>[4x]GLSSSPSEILQELGKGSTHPQPGVSPPAAPAAPGPKDGPGETDAFGNSEGKELVASGENKIKQGLLPSLEDLLFYTIAEGQEKIPVHKFITALKSTGLRTSDPRLKECMDMLRLTLQTTSDGVMLDKDLFKKCVQSNIVLLTQAFRRKFVIPDFMSFTSHIDELYESAKKQSGGK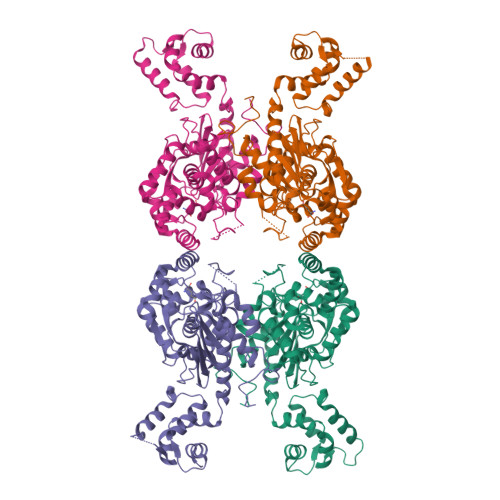VADYIPQLAKFSPDLWGVSVCTVDGQRHSTGDTKVPFCLQSCVKPLKYAIAVNDLGTEYVHRYVGKEPSGLRFNKLFLNEDDKPHNPMVNAGAIVVTSLIKQGVNNAEKFDYVMQFLNKMAGNEYVGFSNATFQSERESGDRNFAIGYYLKEKKCFPEGTDMVGILDFYFQLCSIEVTCESASVMAATLANGGFCPITGERVLSPEAVRNTLSLMHSCGMYDFSGQFAFHVGLPAKSGVAGGILLVVPNVMGMMCWSPPLDKMGNSVKGIHFCHDLVSLCNFHNYDNLRHFAKKLDPRREGGDQRHSFGPLDYESLQQELALKETVWKKVSPESNEDISTTVVYRMESLGEKSHHHHHH>[3x]AQVINTFDGVADYLQTYHKLPDNYITKSEAQALGWVASKGNLADVAPGKSIGGDIFSNREGKLPGKSGRTWREADINYTSGFRNSDRILYSSDWLIYKTTDHYQTFTKIR;>KKA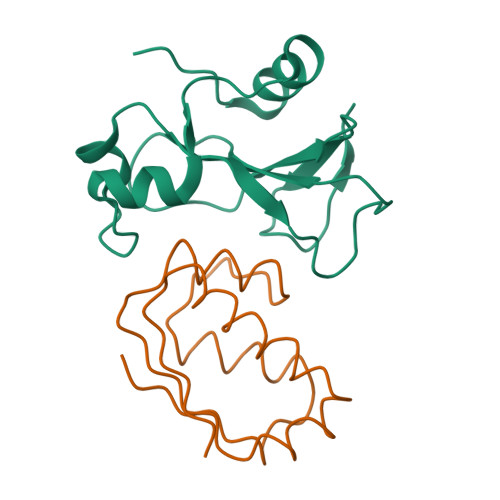VINGEQIRSISDLHQTLKKELALPEYYGENLDALWDALTGWVEYPLVLEWRQFEQSKQLTENGAESVLQVFREAKAEGADITIILS[3x]>[4x]DRHHHHHHGSGPYTKSHGPSHSHRYVRDSQPVAHGTVTHETQAASKHSNSPVLESNIFISDITDDSGTHRWVSGHITEVHDPLRSVSVLEPGGPGGCAHNHRELVEVTAKTRKCLVAQNGGYFDTHTGQCLGNII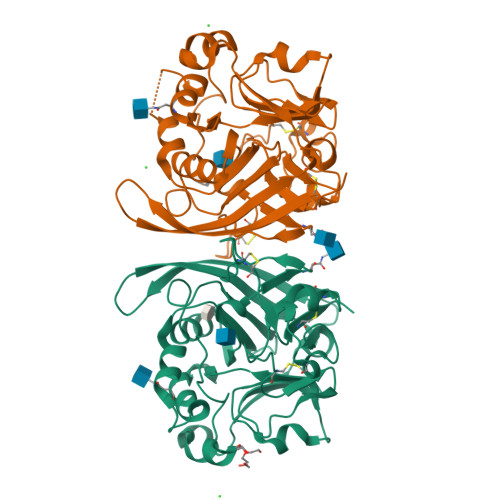SDGKLVRNSGGIQNAQFGIRKDGTLVFGYLSEDDILDQENPFVQLISGVVWLLRKGEIYINESIQAESDKTQETGNFRHFVDVISARTAVGHDKEGKLILFHVDGQTDVRGMNLWQVAKFLKDQNVMNAINLDGGGSATYVLNGSLASYPSDHCNPSKWRCPRAISTVLCIHER2,4-DINITROPHENYL-2-DEOXY-2-FLUORO-BETA-D-CELLOBIOSIDE | C18 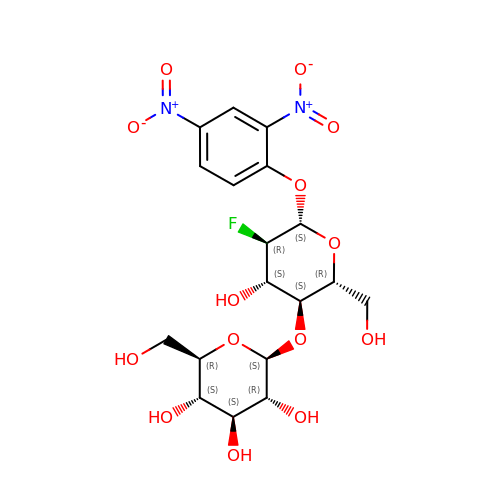H23 F N2 O14 | WFVCNOHOODVBQK-IUBYCILNSA-N> MATLLRSLALFKRNKDKPPITSGSGGAIRGIKHIIIVPIPGDSSITTRSRLLDRLVRLIGNPDVSGPKLTGALIGILSLFVESPGQLIQRITDDPDVSIRLLEVVQSDQSQSGLTFASRGTNMEDEADQYFSHDDPISSDQSRFGWFEN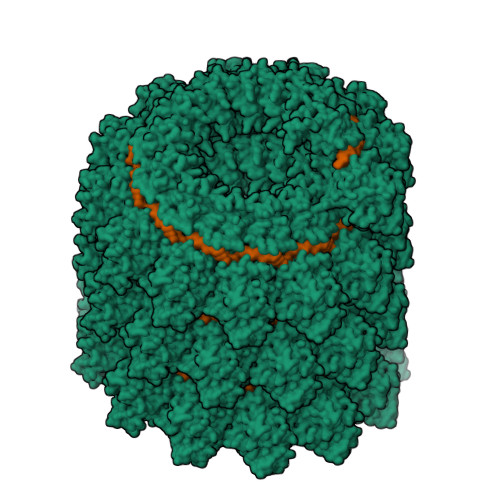KEISDIEVQDPEGFNMILGTILAQIWVLVAKAVTAPDTAADSELRRWIKYTQQRRVVGEFRLERKWLDVVRNRIAEDLSLRRFMVALILDIKRTPGNKPRIAEMICNIDTYIVEAGLASFILTIKFGIETMYPALGLHEFDGELSTLESLMNLYQQMGETAPYMVILENSIQNKFSAGSYPLLWSYAMGVGVELENSMGGLNFGRSYFDPAYFRLGQEMVRRSAGKVSSTLASELGITAEDA>[2x]GSMRHERVVIIKNMFHPMDFEDDPLVLNEIREDLRVECSKFGQ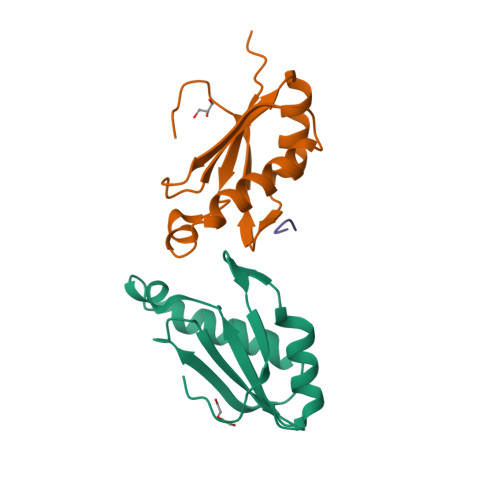IRKLLLFDRHPDGVASVSFRDPEEADYCIQTLDGRWFGGRQITAQAWDGTTDY;> SRWD>[6x]MPTLPKAEAKELSAFVQSCVEYKTNVCFTDVAAYESNQKGVLSSGLAVLVGTHKQLRDPAVQRLPFYNPAVAEAIERVKEGGTYGVLVEGLANAAGSKFVRVVVGEVPTKASRNNCPARPDVVTXLVTAALDE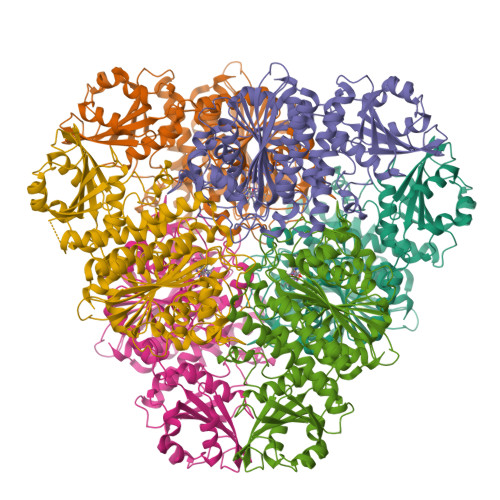VKEPNTTVDVFVLSNAVLPIAAAVARCGKHNFSAKDGAAAAAYNSGKVSRLQVVFPEPPAIPPKDLEAVATSTQLCQRLVDAPPNLLTTATFTEIAQGYAKALGFDVDVICGDDLCERGYGGIYSVGKAAFEAPRLVTLLYTPKGTPVKKVSLVGKGIVYDCGGLALKPADYMKLMKHDMGGAAAVFCGFLTAVRLQQPVQLSCTLCLAENAIGPKSYRNDDIIVMKSGKTVEVINTDAEGRIVLGDGVFHATNELSFTPDVVIDMATLTGAQGIATGRHHAGLYVNEEGAEAAMLRAGRESGETCFPVLYCPEYHEPEFKSNHADMTNLMERRDNAGVSCAGYFITTHLSPKFTGAHIHVDLAYPVFNSNGATGFGPALLTEYFRKL5-HYDROXY-2-(HYDROXYMETHYL)-4H-PYRAN-4-ONE 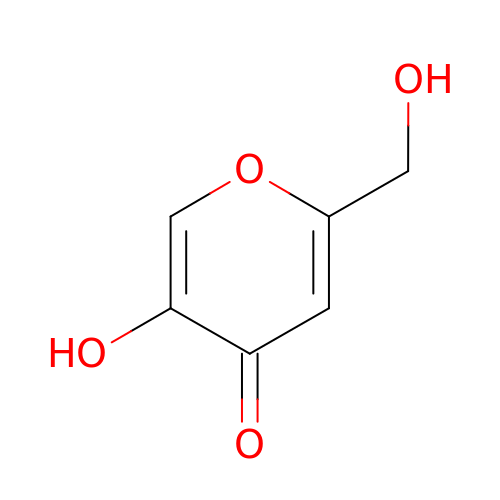| C6 H6 O4 | BEJNERDRQOWKJM-UHFFFAOYSA-N> LPSLEDLLFYTIAEGQEKIPVHKFITALKSTGLRTSDPRLKECMDMLRLTLQTTSDGVMLDKDLFKKCVQSNIVLLTQAFRRKFVIPDFMSFTSHIDELYESAKKQSGGKVADYIPQLAKFSPDLWGVSVCTVDGQRHSIGDTKVPFCLQSCVKPLKYAIAVNDLGTEYVHRYVGKEPSGLRFNKLFLNEDDKPHNPMVNAGAIVVTSLIKQGVNNAEKFDYVMQFLNKMAGNEYVGFSNATFQSERESGKRNFAIGYYLKEKKCFPEGTDMVGILDFYFQLCSIEVTCESASVMAATLANGGFCPITGERVLSPEAVRNTLSLMHSCGMYDFSGQFAFHVGLPAKSGVAGGILLVVPNVMGMMCWSPPLDKMGNSVKGIHFCHDLVSLCNFHNYD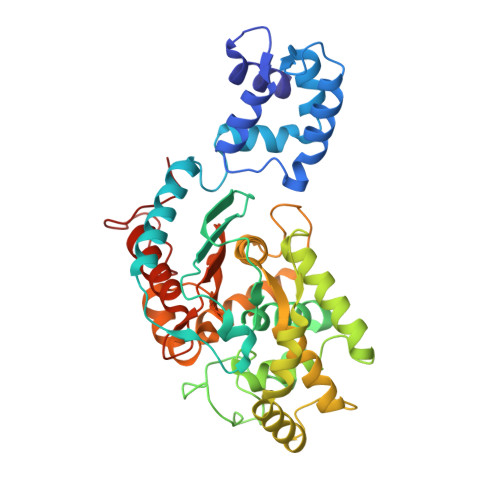NLRHFAKKLDPRREG>SKIGINGFGRIGRLVLRAALSCGAQVVAVNDPFIALEYMVYMFKYDSTHGVFKGEVKMEDGALVVDGKKITVFNEMKPENIPWSKAGAEYIVESTGVFTTIEKASAHFKGGAKKVVISAPSADAPMFVCGVNLEKYSKDMTVVSNASCTTNCLAPVAKVLHENFEIVEGLMTTVHAVTATQKTVDGPSAKDWRGGRGAAQNIIPSSTGAAKAVGKVIPELDGKLTGMAFRVPTPDVSVVDLTVRLGKECSYDDIKAAMKTASEGPLQGFL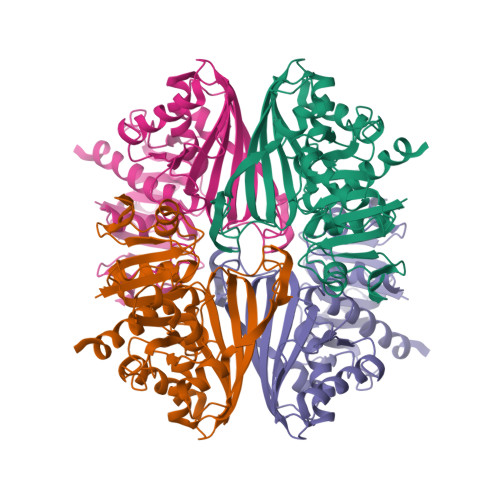GYTEDDVVSSDFIGDNRSSIFDAKAGIQLSKTFVKVVSWYDNEFGYSQRVIDLLKHMQKVDSA[4x]> AAAXDXSLVEVHXXVFIVPPXILQ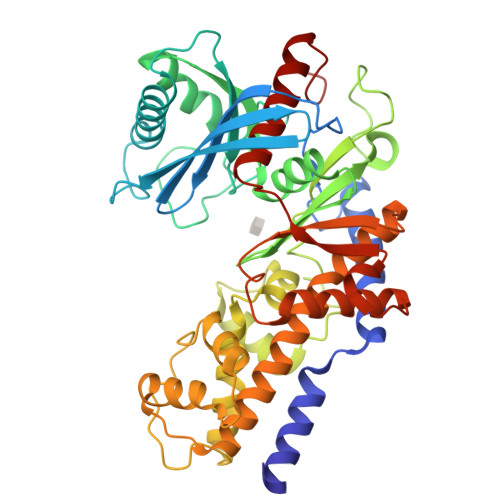AVVSILTTRXDDXDSSAASIPMVPGWVLKQVSGAQAGSFLAIVMGGGDLEVILISLAGRQESSIXASRSLAAAMSTTAIPSDLWGNXAXSNAAFSSXEFSSXAGSVPLGFTFXEAGAKEXVIKGQITXQAXAFSLAXLXKLISAMXNAXFPAGDXXXSVADIXDSHGILXXVNYTDAXIKMGIIFGSGVNAAYWCDSTXIGDAADGGXXGGAGXMXICCDQSSFRKAFPSLPQIXYLXTLNXXSPXAXKTFXKNSXAKNXGQSLRDVLMXFKXXGQXHXXXAXSFXAANVENTSYPAKIQKLPHFDLRXXXDLFXGDQGIAXKTXMKXVVRRXLFLIAAYAFRLVVCXIXAICQKKGYSSGHIAAXGSXRSYSGFSXNSATXNXNIYGWPQSAXXSKPIXITPAIDGXGAASXVIXSIASAXXSXAXXSAXXA> HMN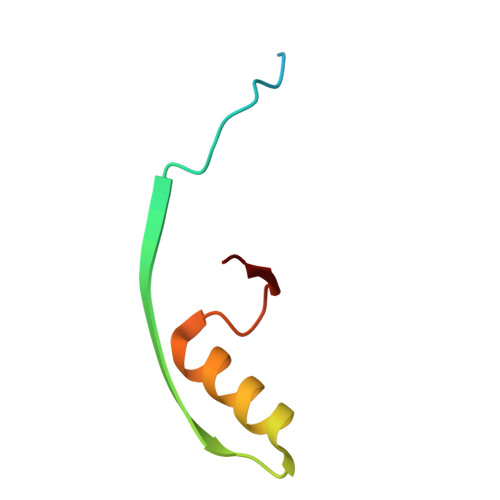AEINPLHAYFKLPNTVSLVAGSSEGETPLNAFDGALLNAGIGNVALIRIS> MTSVNSAEASTGAGGGGSNPVKSMWSEGATFSANSVTCTFSRQFLIPYDPEHHYKVFSPAASSCHNASGKEAKVCTISPIMGYSTPWRYLDFNALNLFFSPLEFQHLIENYGSIAPDALTVTISEIAVKDVTDKTGGGVQVTDSTTGRLCMLVDHEYKYPYVLGQGQDTLAPELPIWVYFPPQYAYLTVGDVNTQGISGDSKKLASEESAFYVLEHSSFQLLGTGGTATMSYKFPPVPPENLEGCSQHFYEMYNPLYGSRLGVPDTLGGDPKFRSLTHEDHAIQPQNFMPGPLVNSVSTKEGDSSNTGAGKALTGLSTGTSQNTRISLRPGPVSQPYHHWDTDKYVTGINAISHGQTTYGNAEDKEYQQGVGRFPNEKEQLKQLQGLNMHTYFPNKGTQQYTDQIERPLMVGSVWNRRALHYESQLWSKIPNLDDSFKTQFAALGGWGLHQPPPQIFLKILPQSGPIGGIKSMGITTLVQYAVGIMTVTMTFKLGPRKATGRWNPQPG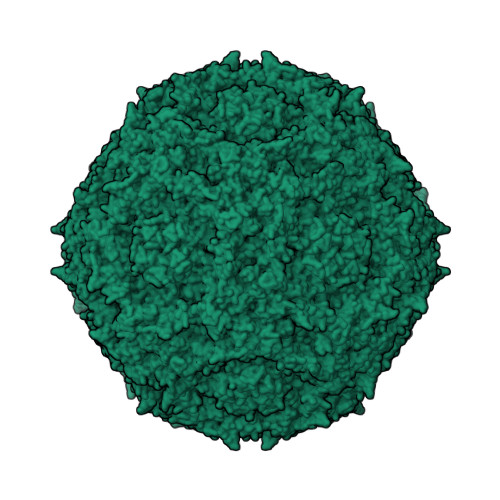VYPPHAAGHLPYVLYDPTATDAKQHHRHGYEKPEELWTAKSRVHPL>[3x]MEIDKELAPQDRTVTVATVLPAVPGPSPLTIKQPFQS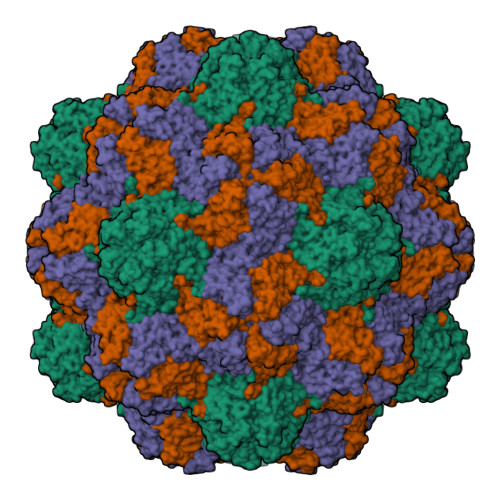EVLFAGTKDAEASLTIANIDSVSTLTTFYRHASLESLWVTIHPTLQAPTFPTTVGVCWVPAQSPVTPAQITKTYGGQIFCIGGAIQTLSPLIVKCPLEMMQPRVKDSIQYLDSPKLLISITAQPTAPPASTCIITVSGTLSMHSPLITDTST[(2R,3S,4R,5R)-5-(2-amino-6-oxo-1,6-dihydro-9H-purin-9-yl)-3,4-dihydroxytetrahydrofuran-2-yl]methyl (2R,3S,4S,5S,6R)-3,4-dihydroxy-5-[({3-hydroxy-2-methyl-5-[(phosphonooxy)methyl]pyridin-4-yl}methyl)amino]-6-methyltetrahydro-2H-pyran-2-yl 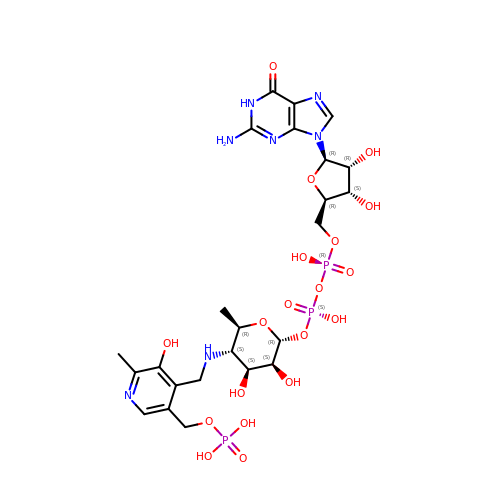dihydrogen diphosphate | C24 H36 N7 O19 P3 | BNJJFFPICXKOFM-VMLLIFSYSA-N HYDANTOCIDIN-5'-PHOSPHATE | C7 H11 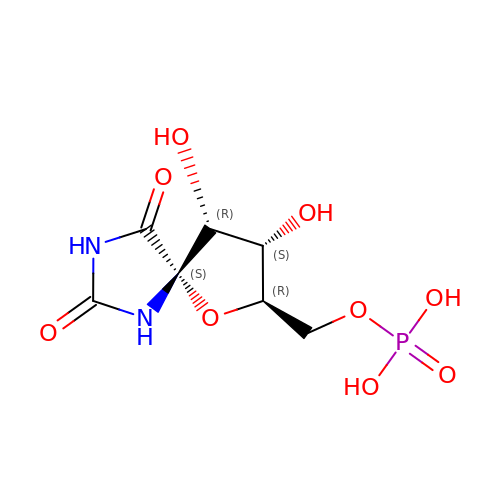N2 O9 P | HVXIMXHBUJADCC-GTBMBKLPSA-N> GPDSMKETPLSNCERRFLLRAIEEKKRLDGRQTYDYRNIRISFGTDYGCCIVELGKTRVLGQVSCELVSPKLNRATEGILFFNLELSQMAAPAFEPGRQSDLLVKL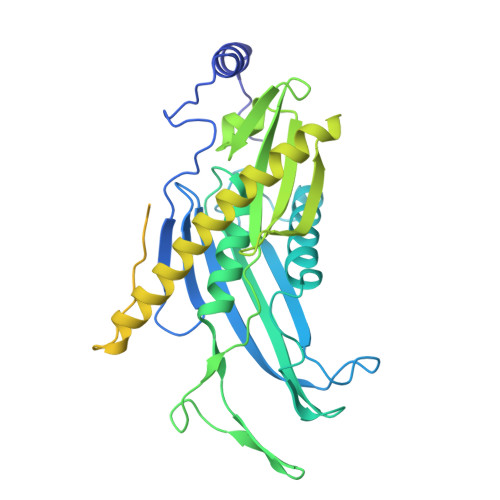NRLMERCLRNSKCIDTESLCVVAGEKVWQIRVDLHLLNHDGNIIDAASIAAIVALCHFRRPDVSVQGDEVTLYTPEERDPVPLSIHHMPICVSFAFFQQGTYLLVDPNEREERVMDGLLVIAMNKHREICTIQSSGGIMLLKDQVLRCSKIAGVKVAEITELILKALENDQKVRKEGGKFGFAESIANQRITAFKMEKAPIDTSDVEEKAEEIIAEAEPPSEVVSTPVLWTPGTAQIGEGVENSWGDLEDSEKEDDEGGGDQAIILDGIKMDTGVEVSDIGSQDAPIILSDSEEEEMIILEPDKNPKKIRTQTTSAKQEKAPSKKPVKRRKKKRAAN> MSSVKISPLKDSEAFQSIKVGNNTLQTKIVYPPTTRFRALEDHTPSDLQLQYYGDRSTFPGTLLITEATFVSPQASGYEGAAPGIWTDKHAKAWKVITDKVHANGSFVSTQLIFLGRVADPAVMKTRGLNPVSASATYESDAAKEAAEAVGNPVRALTTQEVKDLVYETYTNAAQKAMDAGFDYIELHAAHGYLLDQFLQPCTNQRTDEYGGSIENRARLILELIDHLSTIVGADKIGIRISPWATFQNMKAHKDTVHPLTTFSYLVHELQQRADKGQGIAYISVVEPRVSGNVDVSEEDQAGDNEFVSKIWKGVILKAGNYSYDAPEFKTLKEDIADKRTLVGFSRYFTSNPNL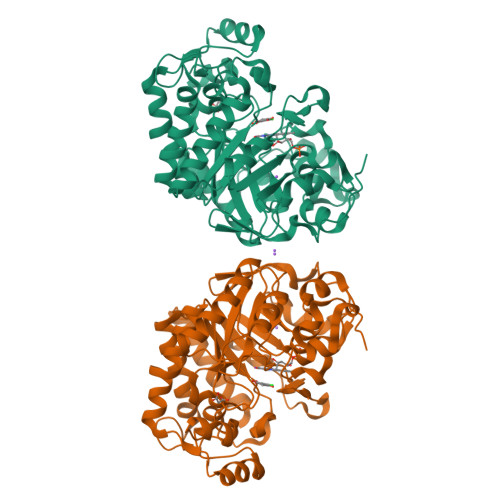VWKLRDGIDLVPYDRNTFYSDNNYGYNTFSMDSEEVDKELEIKRVPSAIEAL>GSHMSNNQTVLPFDGLNYPEGLAVDTQGAVYVAD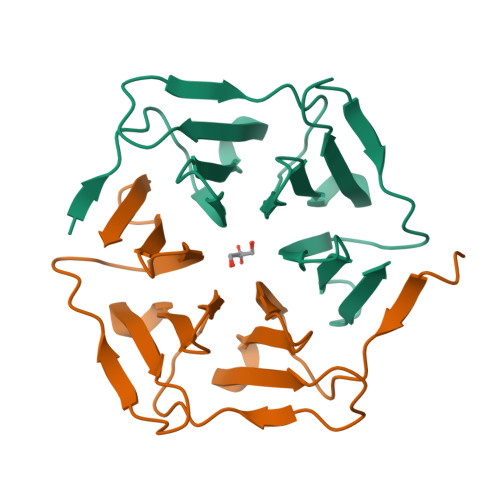RGNNRVVKLAAGSKTQTVLPFTGLNDPDGVAVDNSGNVYVTDTDNNRVVKLEAESNNQVVLPFTDITAPWGIAVDEAGTVYVTEHNTNQVVKLL[2x]> MAAPVVAPPGVVVSRANKRSGAGPGGSGGGGARGAEEEPPPPLQAVLVADSFDRRFFPISKDQPRVLLPLANVALID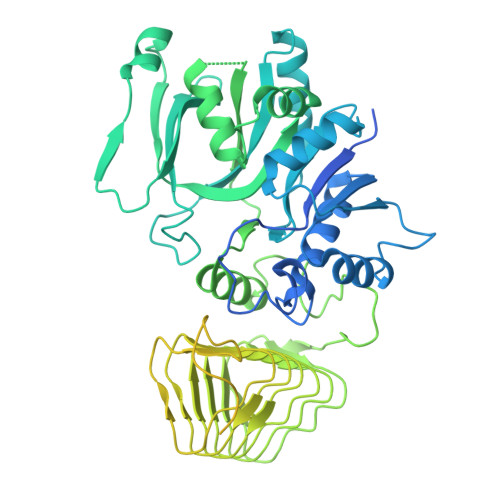YTLEFLTATGVQETFVFCCWKAAQIKEHLLKSKWCRPTSLNVVRIITSELYRSLGDVLRDVDAKALVRSDFLLVYGDVISNINITRALEEHRLRRKLEKNVSVMTMIFKESSPSHPTRCHEDNVVVAVDSTTNRVLHFQKTQGLRRFAFPLSLFQGSSDGVEVRYDLLDCHISICSPQVAQLFTDNFDYQTRDDFVRGLLVNEEILGNQIHMHVTAKEYGARVSNLHMYSAVCADVIRRWVYPLTPEANFTDSTTQSCTHSRHNIYRGPEVSLGHGSILEENVLLGSGTVIGSNCFITNSVIGPGCHIGDNVVLDQTYLWQGVRVAAGAQIHQSLLCDNAEVKERVTLKPRSVLTSQVVVGPNITLPEGSVISLHPPDAEEDEDDGEFSDDSGADQEKDKVKMKGYNPAEVGAAGKGYLWKAAGMNMEEEEELQQNLWGLKINMEEESESESEQSMDSEEPDSRGGSPQMDDIKVFQNEVLGTLQRGKEENISCDNLVLEINSLKYAYNVSLKEVMQVLSHVVLEFPLQQMDSPLDSSRYCALLLPLLKAWSPVFRNYIKRAADHLEALAAIEDFFLEHEALGISMAKVLMAFYQLEILAEETILSWFSQRDTTDKGQQLRKNQQLQRFIQWLKEAEEESSEDD> GSHMVEIIPVSTTLELRAADESHVPALHQLVLKNKAWLQQSLDWPQYVTSQEETRKHVQGN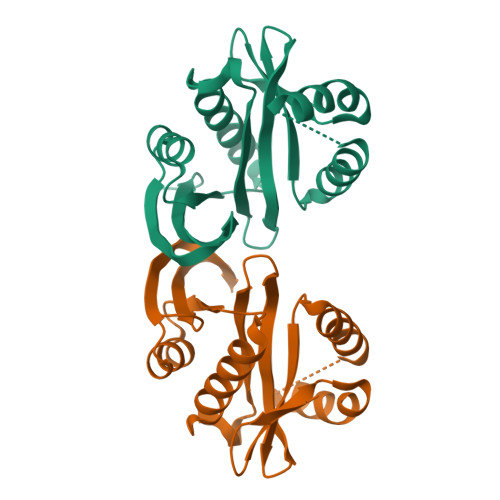ILLHQRGYAKMYLIFCQNEMAGVLSFNAIEPINKAAYIGYWLDESFQGQGIMSQSLQALMTHYARRGDIRRFVIKCRVDNQASNAVARRNHFTLEGCMKQAEYLNGDYHDVNMYARIIDAD>[2x]GDTHEFHKLLIKVVDLFLEDRIKEFELKLNTTLDELEFEELIGKPDSSNSAENNGIF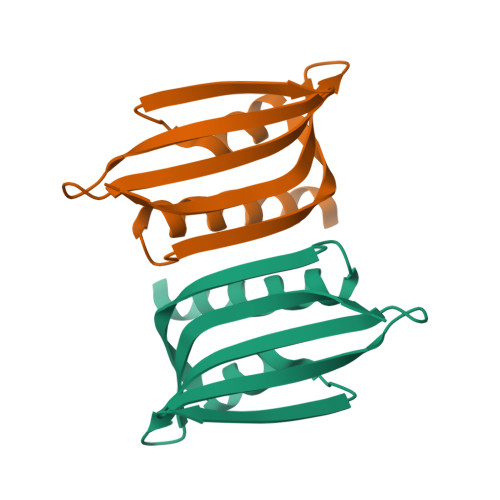IDEYSYDASENAIKKLFVEYVRQPEFKYTVLSIKGVNDWVRE> MEWSQIFHDITTKHDFKAMHDFLEKEYSTAIVYPDRENIYQAFDLTPFENIKVVILGQDPYHGPNQAHGLAFSVQPNAKFPPSLRNMYKELADDIGCVRQTPHLQDWAREGVLLLNTVLTVRQGEANSHRDIGWETFTDEIIKAVSDYKEHVVFILWGKPAQQKIKLIDTSKHCIIKSVHPSPLSAYRGFFGSKPYSKANTYLESVGKSPINWCESEALEHHHH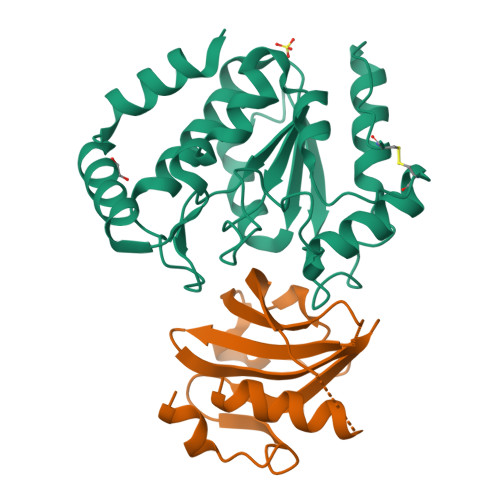HH;> MKQIKAHLTRYLEEILKLSSQEYLTEFVQLGIEELAWGERKIPEKLKGAIIDTYTFYDHSLIKDYIYSFIGTYQGKIILVGYTNGEYEHFFYINDTVKTLHSELHLLNLTEEDLEFVNVG>[4x]MGETMSKRLKLHLGGEAEMEERAFVNPFPDYEAAAGALLASGAAEETGCVRPPATTDEPGLPFHQDGKIIHNFIRRIQTKIKDLLQQMEEGLKTADPHDCSAYTGWTGIALLYLQLYRVTCDQTYLLRSLDYVKRTLRNLNGRRVTFLCGDAGP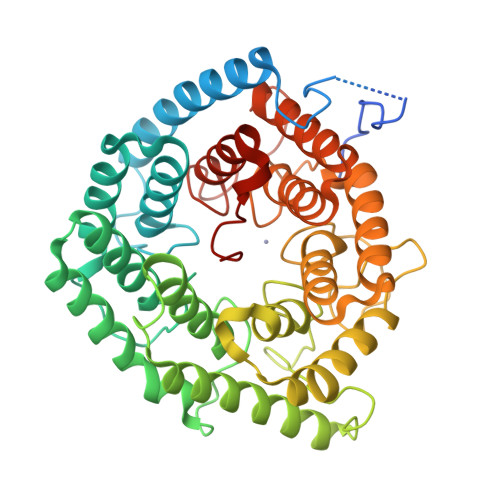LAVGAVIYHKLRSDCESQECVTKLLQLQRSVVCQESDLPDELLYGRAGYLYALLYLNTEIGPGTVCESAIKEVVNAIIESGKTLSREERKTERCPLLYQWHRKQYVGAAHGMAGIYYMLMQPAAKVDQETLTEMVKPSIDYVRHKKFRSGNYPSSLSNETDRLVHWCHGAPGVIHMLMQAYKVFKEEKYLKEAMECSDVIWQRGLLRKGYGICHGTAGNGYSFLSLYRLTQDKKYLYRACKFAEWCLDYGAHGCRIPDRPYSLFEGMAGAIHFLSDVLGPETSRFPAFELDSSKRD> MANSLEPEPWFFKNLSRKDAERQLLAPGNTHGSFLIRESESTAGSFSLSVRDFDQNQGEVVKHYKIRNLDNGGFYISPRITFPGLHEL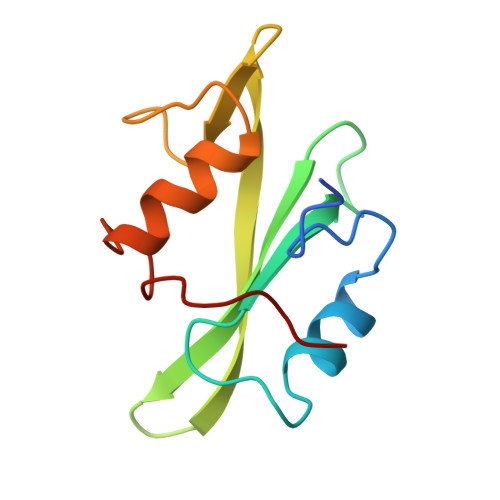VRHYTNASDGLCTRLSRPCQT2-azanyl-5-phenyl-3-(4-sulfamoylphenyl)benzamide | C19 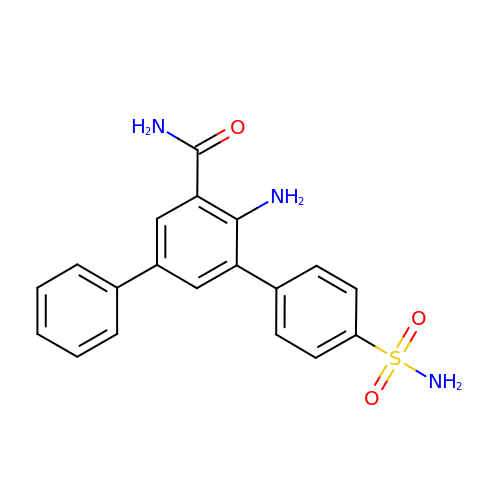H17 N3 O3 S | IVJPEEHVYKDQEO-UHFFFAOYSA-N PL kinase is one of the key enzymes involved in PLP metabolism. In the presence of MgATP, this enzyme catalyzes the phosphorylation of the three inactive primary forms of vitamin B6, i.e. pyridoxine (PN), pyridoxamine (PM), and pyridoxal (PL) to their 5′-phosphorylated forms, PNP, PMP and PLP, respectively. PL kinase is a homodimer with each active site exclusively formed by a single monomer. The ATP binds in a shallow cavity at the active site, while the vitamin B6 substrate binds in a solvent-inaccessible deeper cavity opposite but facing the γ-phosphate of the ATP.

Theophylline is bound at the PL binding site in both subunits, with an occupancy of 60%. Occupying the same position as the theophylline is a 2-methyl-2,4-pentanediol (MPD) molecule at 40% occupancy. Possible contacts between the active site residues and theophylline involve a hydrogen-bond interaction between the hydroxyl group of Ser12 and the N9 of the theophylline imidazole nitrogen, which is also present between Ser12 and the pyridine nitrogen atom of PM in the sheep PL kinase structure. In the theophylline complex, the C6 oxygen of the piperazine ring and the N7 of the imidazole ring are adjacent to Thr47, but any possible hydrogen-bond interactions are considerably lengthened beyond 3.6 Å. In the sheep structure, Asp235 makes a strong hydrogen-bond interaction with the C5′-OH group of PM. This interaction is conserved with the C2 oxygen of theophylline. In addition the C2 oxygen atom is involved in water-mediated interactions with the side-chains of Asp235, Gln11 or main-chain nitrogen of Tyr84. Both PM and theophylline make hydrophobic interactions with the protein residues Val231, Val19, Tyr84 and Phe43. A bound Na+ in the hPL kinase-theophylline structure is located at the ATP binding site, and is coordinated by five well-defined water molecules. The intricate water-mediated interaction between the Na+ and the protein is believed to stabilize the active site conformation. Detailed kinetic studies with ginkgotoxin, theophylline, lamotrigine and enprofylline showed the compounds to inhibit hPL kinase with a Ki of 3, 50, 56 and 228 µM, repectively.

>[2x]MEEECRVLSIQSHVIRGYVGNRAATFPLQVLGFEIDAVNSVQFSNHTGYAHWKGQVLNSDELQELYEGLRLNNMNKYDYVLTGYTRDKSFLAMVVDIVQELKQQNPRLVYVCDPVLGDKWDGEGSMYVPEDLLPVYKEKVVPLADIITPNQFEAELLSGRKIHSQEEALRVMDMLHSMGPDTVVITSSDLPSPQGSNYLIVLGSQRRRNPAGSVVMERIRMDIRKVDAVFVGTGDLFAAMLLAWTHKHPNNLKVACEKTVSTLHHVLQRTIQCAKAQAGEGVRPSPMQLELRMVQSKRDIEDPEIVVQATVL>MSADVAGAVIDGAGLGFDVLKTVLEALGNVKRKIAVGIDNESGKTWTAMNTYFRSGTSDIVLPHKVAHGKALLYNGQKNRGPVATGVVGVIAYSMSDGNTLAVLFSVPYDYNWYSNWWNVRVYKGQKRADQRMYEELYYHRSPFRGDNGWHSRGLGYGLKSRGFMNSSGHAILEIHVTKA[2x]

Fragaceatoxin C (FraC)11 is a potent haemolysin of the family of actinoporins, defined as a group of ~20 kDa protein toxins produced by sea anemones. Actinoporins are classified as α-helical PFT (α-PFT) because the transmembrane pore is predicted to form an α-helical barrel. The lytic activity of actinoporins on biological membranes is enhanced by the lipid sphingomyelin (SM) and by lipid-phase coexistence. Here we reveal structures of FraC corresponding to four different stages of its activation route, namely the water-soluble form, the lipid-bound form, an assembly intermediate and the transmembrane pore.

In the monomeric form of FraC, the side chain of Phe16 is inserted in a hydrophobic cavity of the β-core region.> ATDVATVVSQAKAQMKEAYYTYSHTVTETGQFPDIKDVYAAYNKAKQAYANAVAVVNKAGGAKKDAYLADLQAIYETYVFKANPKSGEARVATYIDAYNYATKLDKMRQELKAAVDAKDLKKAEELYHKISYELKTRTVILDRVYGQSTRELLRSTFKADAQALRDRLIYDITVAMKAREAQDAVKAGNLDKAKAALDQVNQYVSKVTDAFKAELQKAAQDAKAAYEAALTPKVESVSAIDSTSFKVTFTKPVDKATAIPKNFSITLKGTETKLYPKSVEVSESGLTATVTLYDTLVDGKTYTVVTSGLKDTAGKEFETSTNEFTYNKPVPASITFNFNKLPEDSAVDLTKYVTVKDAAGNVIKSGFELEFTSSEKLTQGKFINTTGKKSVIVNATVKGTNVTTGNVILAVEDEKAAEVSELKLTKDNKEVVTLYANGNAFDKDGNQISSGTLTLTAKFKDQYGNELTGKVAGTDYTFESLNPEVLVVAPDGSVTPIVPGTALVKVKYGEVTKTIPVTVKANPVLETIAVDSTGVSVAKGQKATFKV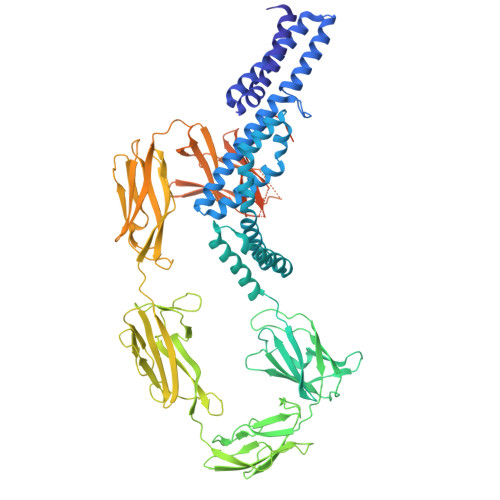TLKDQYGNKFTGNVNVTSDKTETATVSVSNSGIGQSEYTVTVNGVAEGSTTITIKSGTKEVKVPVNVVAGGPVANYQIKVLDDGKIDKSATESPANNDVQLKVYAVDANGNIVGDITNDVTITSEATDTNGVIVNASKSTANGDTVYVITDNGSKKVGKETLTVKLGTVTLGTVDVEVIDTTLKATVVTKKADLIELDAADNGDALAKLLANLDIKDQNGNPMVDSAATPNTNEKLQALKSVLSGIVSSDTSVIGSVSNVDNLKDDA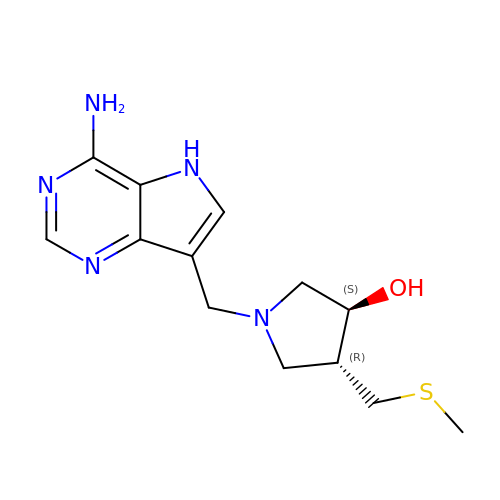(3S,4R)-1-[(4-amino-5H-pyrrolo[3,2-d]pyrimidin-7-yl)methyl]-4-[(methylsulfanyl)methyl]pyrrolidin-3-ol | C13 H19 N5 O S | NTHMDFGHOCNNOE-VHSXEESVSA-N5-fluoro-1-(beta-D-glucopyranosyl)pyrimidine-2,4(1H,3H)-dione | C10 H13 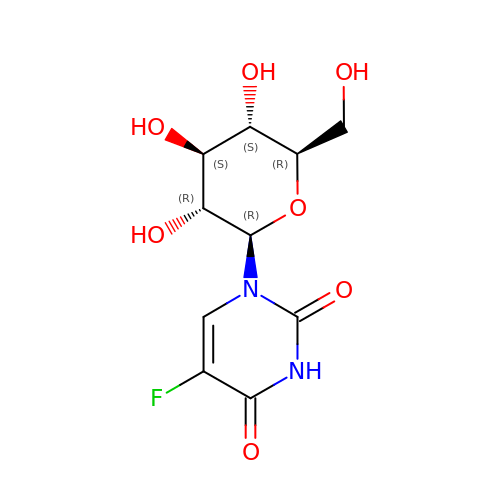F N2 O7 | YHWGRVDTEORPPJ-XSEHCYKFSA-N> LKESPSGYLRSGEGDTGCGELVWVGEPLTLRTAETI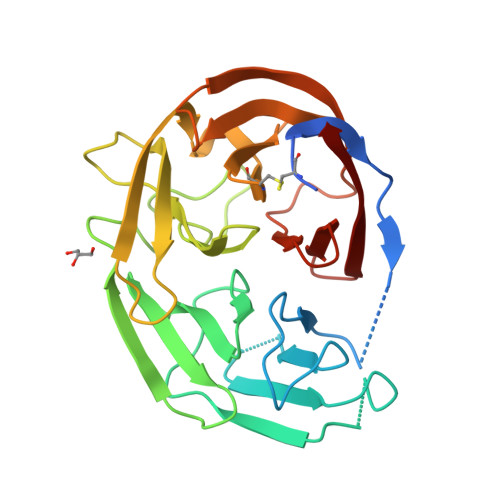TGKYGVWMRDPKPTYPYTQETTWRIDTVGTDVRQVFEYDLISQFMQGYPSKVHILPRPLESTGAVVYSGSLYFQGAESRTVIRYELNTETVKAEKEIPGAGYHGQFPYSWGGYTDIALAVDEAGLWVIYSTDEAKGAIVLSKLNPENLELEQTWETNIRKQSVANAFIICGTLYTVSSYTSADATVNFAYDTGTGISKTLTIPFKNRYKYSSMISYNPLEKKLFAWDNLNMVTYDIKLSKM> MKDIGIVGYGSYIPKYRIKVEEIAKVWGKDPEAIKKGLVVNEKSVPSPDEDTATIAVEAARNAVKRAGINAEKIGAVYVGSESHPYAVKPTSATVAEAIGATPDLTAADLEFA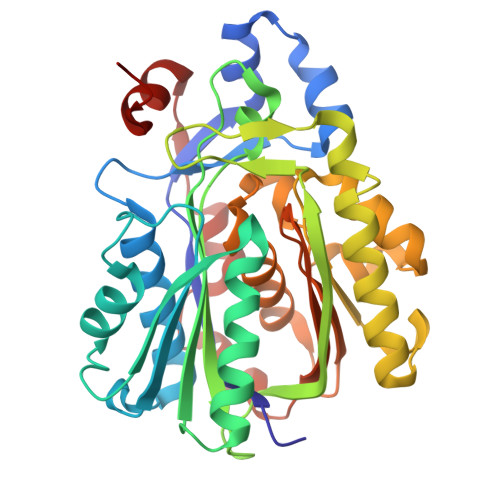CKAGTAGIQMCMGLVGSGLIEYGMAIGADTAQGAPGDALEYTASAGGAAYIIGNKKDEMIAVFNGTYSYTTDTPDFWRREGQSYPKHGGRFTGEPAYFKHVLNAAKGIMEKMGTTVKDYDYCVFHQPNGKFYIKAAKSLGFTNEQYKYGLLTPYLGNTYSGAVPLGLSNILDHAEEGARILAVSYGSGAGSDAFDITVTERIKEVVDKAPKTLDLLNRKKYIDYAVYVKYRGKIKI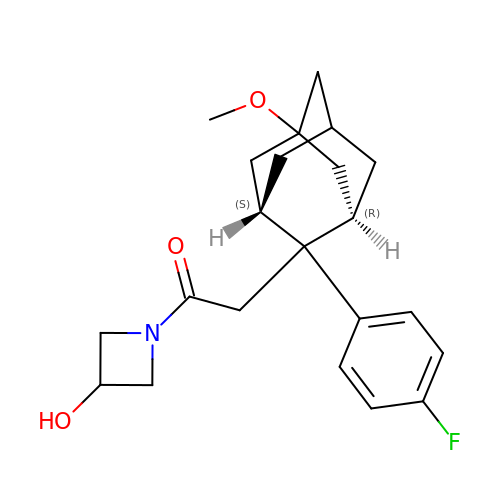1-(3-HYDROXYAZETIDIN-1-YL)-2-[(2S,5R)-2-(4-FLUOROPHENYL)-5-METHOXYADAMANTAN-2-YL]ETHAN-1-ONE | C22 H28 F N O3 | AVSPWVIWVZFZOT-GREYGWINSA-N methyl 4-[5,6-bis(chloranyl)-1H-indol-3-yl]-3-(5-chloranyl-1H-indol-3-yl)-1H-pyrrole-2-carboxylate 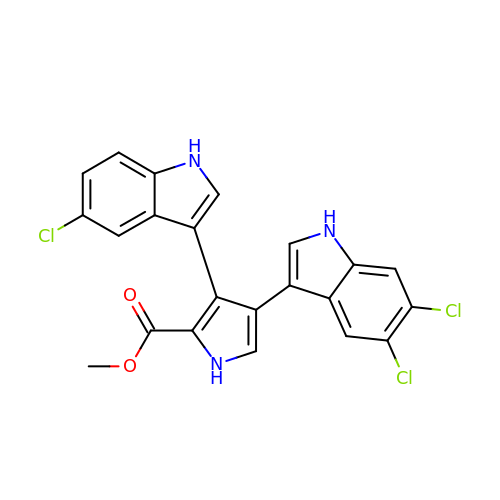| C22 H14 Cl3 N3 O2 | HJXJUNZGSRTQEN-UHFFFAOYSA-N>[2x]QQARQNLQNLYINRC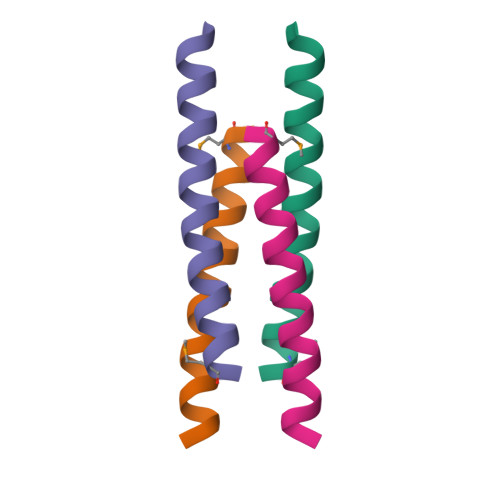LREICQELKEIRAML> SKQDQETYLETIKDFQPTELFQVLATSEDLSIDELLRDSLESYSQDRDRFLQEFINLLLCCCGAIARLEVHDVHSNESSNETVGELQLLFQRQKVHEFHLLISKDSKKKSKYPPLYANFVEFMFRLMDVANDLQLLYVESDEDESEIGTGPLIIDLLTWLSPLSVCKIRSLRYIATLTLYLFQDFLTDHVVDLDKNYLSKLSKQLSVENKKKRPNGKTVEKLESTIAEIQSSKMVTQGIIDNIIKLCFVHRFKDVDETIRCESMVHLASWTKSFPEYFLKVTFLKYFGWLLSDSSVTVRLQVLKILPQLISQHHNRAVDNSAVRQFFERFKERILEIALKDSNLEVRLSAVQVLVEVASLGYLEDTEILSISSLIFEDNEIKVSSLGKNSRYLASVAKFFACITEEKFQEFTNNRVLPKELFDVKGSSAVRIGIFMNLLNESLTEYLQKVPQIGSEKRIHILFQAAEFLYPYFGSLIKDICKVLTFEGEFTHESLETPTYTGDNNNEENNDENNRSNLLLPTDSNNIILYVTTLHGLAYGGTHMRGQPKFKVAEAVLPHLDQLIKRLPIESSNVLASILGVFNLFAFEDWIHTGYEKDIRKILEKIIKAFNESTLTSGAQDLKYKSFSETVSQVRKLGFNELDELWLNHISQLKIHLGKFLEEKLHPDVQDTENDENMNTLYGVFLNKLALLGKVYPIEFQENLLSLFLNRFVQRLPQIGVHCQLETIQEIHLKLLALLTTWQLQKWVDILEKSSENDSPSPVSEFSLRTVSSIVKSFKVIFDALSSDTNDNDGTLGDFLLKWSTSNSFIDIIISLKVFELGVAESEKSWRHALRENFVPYVTDSANQVLLKVFLYLESLFANESSEHLDRNPQEDVNLNDIKYDGFGDGCEKELLLFTIKLKGLMKLGLLDEALFSRIALNKEKLGPLYAKVIEDTIFDQDKKGRVPHHHHHH

Sister chromatid cohesion involves entrapment of sister DNAs by a cohesin ring created through association of a kleisin subunit (Scc1) with ATPase heads of Smc1/Smc3 heterodimers. Cohesin’s association with chromatin involves subunits recruited by Scc1: Wapl, Pds5, and Scc3/SA, in addition to Scc2/4 loading complex. Because all eukaryotic genomes encode orthologs, Scc3 is the most important of cohesin’s regulatory subunits. It has roles in loading of cohesin onto chromosomes as well as its subsequent release.

To obtain the structure of a more complete version of the protein, we expressed Scc3 trimmed of its N- and C-terminal extensions from other yeast species. Of these, Scc3 containing residues 88–1035 from Zygosaccharomyces rouxii (Zr Scc3) yielded crystals suitable for crystallography. Diffraction data were obtained to a resolution of 2.6 Å from crystals grown at pH 6.5 in a PEG/KSCN condition and their structure solved by selenomethionine single-wavelength anomalous dispersion (SAD). The crystal structure of Zr Scc3 reveals a long, partly twisted and partly crescent-shaped protein composed entirely of α-helices stacked on each other in a surprisingly irregular manner, given the repeat nature of the protein. In addition to a pronounced hook within the protein’s C-terminal half, a striking feature is a “nose” at the N-terminal end, a morphology generated by a pair of anti-parallel helices that are about twice as long as their neighbors. At the tip of the nose reside three conserved basic residues, KKR (298–300). Though part of this conserved and essential surface (‘CES’) is positively charged, it also contains numerous conserved aromatic residues, namely Zr H337, F339, Y373, W376, and F417. The highly conserved positively charged residues Zr K340, K372, and R416 all protrude from the surface in a conspicuous manner. Though S. cerevisiae Scc3 packed tightly as dimers in the crystals, those from Z. rouxii crystallized as monomers.>[2x]MPHTLWMVWVLGVIISLSKEESSNQASLSCDRNGICKGSSGSLNSIPSGLTEAVKSLDLSNNRITYISNSDLQRCVNLQALVLTSNGINTIEEDSFSSLGSLEHLDLSYNYLSNLSSSWFKPLSSLTFLNLLGNPYKTLGETSLFSHLTKLQILRVGNMDTFTKIQRKDFAGLTFLEELEIDASDLQSYEP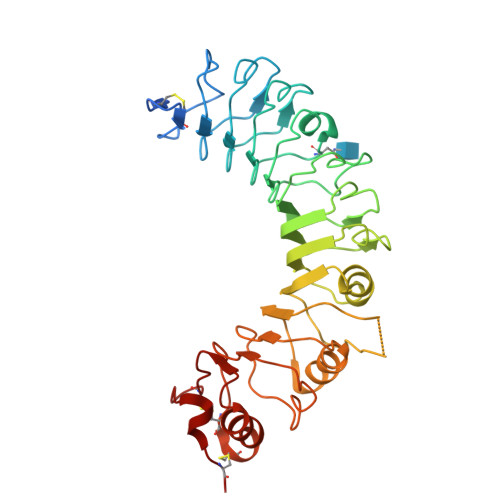KSLKSIQNVSHLILHMKQHILLLEIFVDVTSSVECLELRDTDLDTFHFSELSTGETNSLIKKFTFRNVKITDESLFQVMKLLNQISGLLELEFSRNQLKSVPDGIFDRLTSLQKIWLHTNPWDCSCPRIDYLSRWLNKNSQKEQGSAKCSGSGKPVRSIICP> AERPTLPIPDLLTTDARNRIQ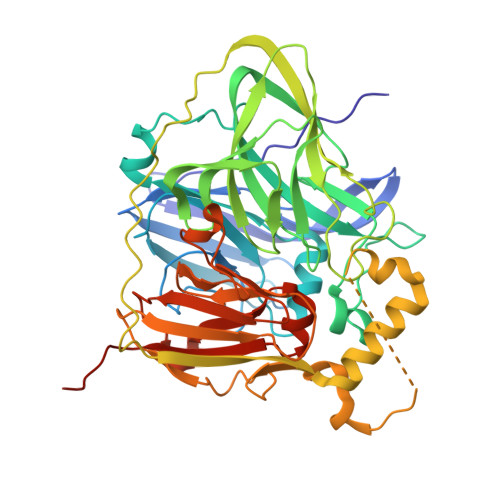LTIGAGQSTFGGKTATTWGYNGNLLGPAVKLQRGKAVTVDIYNQLTEETTLHWHGLEVPGEVDGGPQGIIPPGGKRSVTLNVDQPAATCWFHPHQHGKTGRQVAMGLAGLVVIEDDEILKLMLPKQWGIDDVPVIVQDKKFSADGQIDYQLDVMTAAVGWFGDTLLTNGAIYPQHAAPRGWLRLRLLNGCNARSLNFATSDNRPLYVIASDGGLLPEPVKVSELPVLMGERFEVLVEVNDNKPFDLVTLPVSQMGMAIAPFDKPHPVMRIQPIAISASGALPDTLSSLPALPSLEGLTVRKLQLSMDPMLDMMGMQMLMEKYGDQAMAGMDHSQMMGHMGHGNMNHMNHGGKFDFHHANKINGQAFDMNKPMFAAAKGQYERWVISGVGDMMLHPFHIHGTQFRILSENGKPPAAHRAGWKDTVKVEGNVSEVLVKFNHDAPKEHAYMAHCHLLEHEDTGMMLGFTVLQGDHGLSAWSHPQFEK>[2x]GSWSVKELEDKNEELLSEIAHLKNEVARLKKLLQRCLAANQELRDAIRQSNQILRERAEELLHFQAS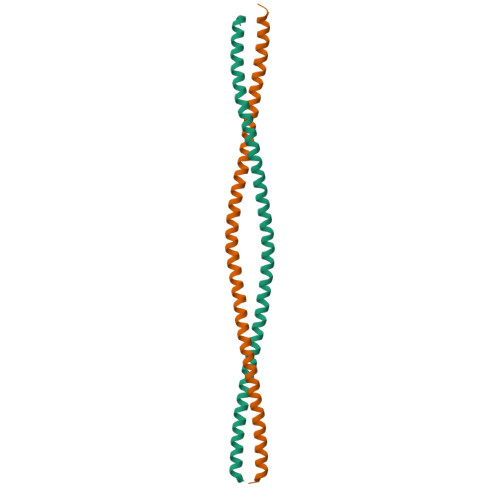QREEKEFLMSKFQEARKLVERLGLEKLELEDKNEELLSEIAHLKNEVARLKKLVGER> GSHMAEKPHMNLVVIGHVDHGKSTLVGHLLYRLGYIEEKKLKELEEQAKSRGKESFKFAWILDKMKEERERGITIDLTFMKFETKKYVFTIIDAPGHRDFV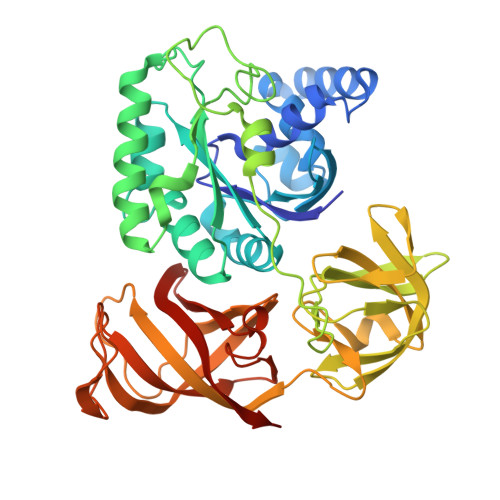KNMITGASQADAAILVVSARKGEFEAGMSTEGQTREHLLLARTMGIEQIIVAVNKMDAPDVNYDQKRYEFVVSVLKKFMKGLGYQVDKIPFIPVSAWKGDNLIERSPNMPWYNGPTLVEALDQLQPPAKPVDKPLRIPVQNVYSIPGAGTVPVGRVETGVLRVGDKVVFMPPGVVGEVRSIEMHYQQLQQAEPGDNIGFAVRGVSKSDIKRGDVAGHLDKPPTVAEEFEARIFVIWHPSAITVGYTPVIHVHTASVSSRIIEIKAKLDPKTGQVVEQNPQFLKAGDAAIVRFKPVKPLVVEKFSEIPQLGRFAMRDMNRTVGIGIVTDVKPAKVDIKAK>[4x]SNAMTVLDREQVLSAFKNRKSCRHYDAARKISAEDFQFILELGRLSPSSVGSEPWQFVVVQNPEIR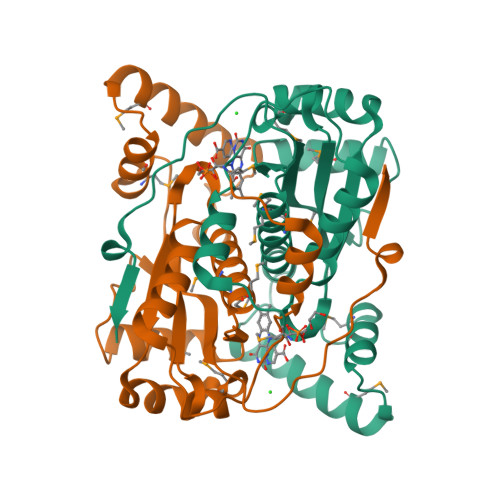QAIKPFSWGMADALDTASHLVVFLAKKNARFDSPFMLESLKRRGVTEPDAMAKSLARYQAFQADDIKILDDSRALFDWCCRQTYIALGNMMTGAAMAGIDSCPVEGFNYADMERVLSGQFGLFDAAEWGVSVAATFGYRVQEIATKARRPLEETVIWA> GSHMAGLP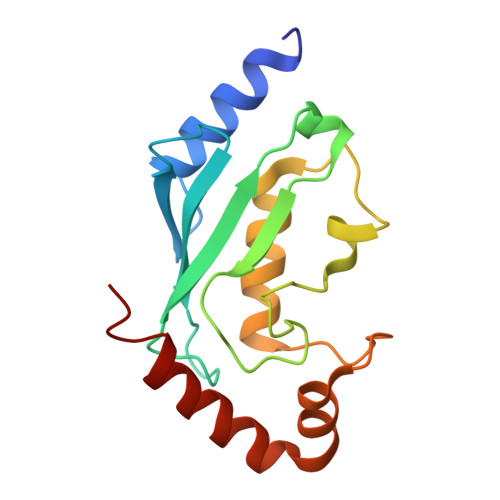RRIIKETQRLLAEPVPGIKAEPDESNARYFHVVIAGPQDSPFEGGTFKLELFLPEEYPMAAPKVRFMTKIYHPNVDKLGRICLDILKDKWSPALQIRTVLLSIQALLSAPNPDDPLANDVAEQWKTNEAQAIETARAWTRLYAMNNI> GMNKMKKVLMTMFGLVMLPLLFACSNNQSAGIEAIKSKGKLVVALNPDFAPFEYQKVVDGKNQIVGSDIELAKAIATELGVELELSPMSFDNVLASVQSGKADLAISGVSKTDERSKVFDFSTPYYTAKNKLIVKKSDLATYQSVNDLAQKKVGAQKGSIQETMAKDLLQNSSLVSLPKNGNLITDLKSGQVDAVIFEEPVAKGFVENNPDLAIADLNFEKEQDDSYAVAMKKDSKELKEAVDKTIQKLKESGELDKLIEDAFKASI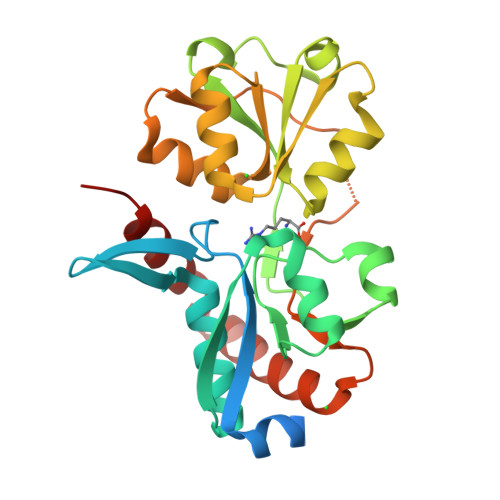EK> MWHYTSINNDTRVALDPKPNQIRTITKPNTVPQLGTDYLYTFNSQRRSHTLRLLGPFQYFNFSETDRGHPLFRLPLKYPSKAIPADELIDNLHSWMRSVHLLHVRSEDNTLRYNWMLGVYARSTNYTTPVGQLVVNAPAILNYSNPQDAFNSVFVALGIDYIDIPITNSNIFDDSSTPYNVRIWHAPTMTEVNHILALMRKSTLVSTHSSWHWDVLHTFHYRSESDMIDHFAAKILEDWRQKEKLDKGALVEADRVVQRLIPLSSSTYVQRLAAIGALYPNEFTENVLDLSRLSTALLQLSDTYYQHANDQLRRLYRRMYNDSRTLYMTQRHQELLLAQITADPNILLYPYTYIFTTAYTSMNYISNTGQGRIKHSLAVTGTTEHTIADITLGPMSEDVVTISMVEPMSIAAEDMYGYVLDTPTRDIWPADEQIEQKGDAVALYDTKTSRALGMFNNTVRIDDLLSPLLGLVYRTYIKGDTMTMTQGSLDHLTLCAAVDSDITFVGNRMIAPLAEGYIPKAMHRNNSTMKMLSLYVALKKLENFTTNSYLMAPDTSIILLGAEREPAVSILRRFNRSVSNVRIIGMGDRAVEPNIRVRVPFPIDKNISADFIICDINSYEDQSFESMFGETISVVTTCASAATRVLVKINHPSEYMINSVIERLSQLGGVFYHTALLKTASQNPYSYETYIYITPIAAAVRFPFYSNSAIINRYMTAVADDETPIIPSIHTVIKGHSNTYSPGLFCGCIDVQSAPFALSQLKSYCSEATTWRVDSDDNLVNIIARIDPARIALEFRTRSNTSAYHEYQRYVPNGLGFKGRKTREFRYIHREVTFIHKLMTYALIREQIS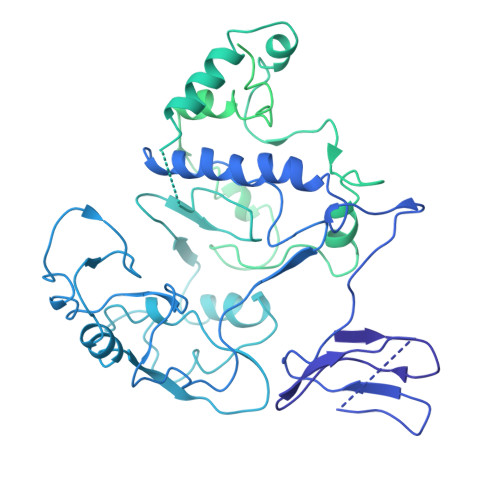LTENMTQVVSIGGRNLADISVVPLNMKYVVIDPATRIETLTQEKKNIEVQSRPFSFDAASMDLENNSIYLFIAVIMNEPNGAATPARTQMDKIRNVATAMLTRTNCVAYISFYEAGIITRLDQSTAHKTIRVEEGRLKVANYVPVDTLVEADVTLMLRDIGITHEIIRPSTPELINACSNYGIRLGSTGGAVLDVFNHYSPVIKLVRS>[4x]GHMKLKTKTMEWSGNSLKLLDQRKLPFIEEYVECKTHEEVAHAIKEMIVRGAPAIGVAAAFGYVLGLRDYKTGSLTDWMKQVKETLARTRPTAVNLFWALNRMEKVFFENADRENLFEILENEALKMAYEDIEVNKAIGKNGAQLIKDGSTILTHCNAGALATVDYGTALGVIRAAVESGKRIRVFADETRPYLQGARLTAWEL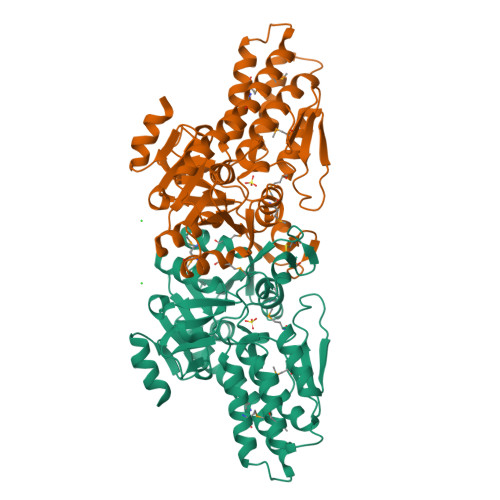MKDGIEVYVITDNMAGWLMKRGLIDAVVVGADRIALNGDTANKIGTYSLAVLAKRNNIPFYVAAPVSTIDPTIRSGEEIPIEERRPEEVTHCGGNRIAPEGVKVLNPAFDVTENTLITAIITEKGVIRPPFEENIKKILEVGS4-{4-(1-methyl-1H-pyrazol-4-yl)-1-[2-(4-methyl-1H-1,2,3-triazol-1-yl)ethyl]-1H-imidazol-5-yl}benzonitrile | C19 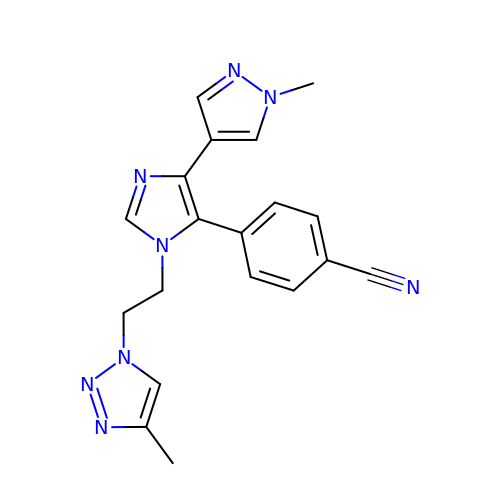H18 N8 | YPRKVQKJNRKXFN-UHFFFAOYSA-N> AFQETNPPAGPVRAIAEYERSAA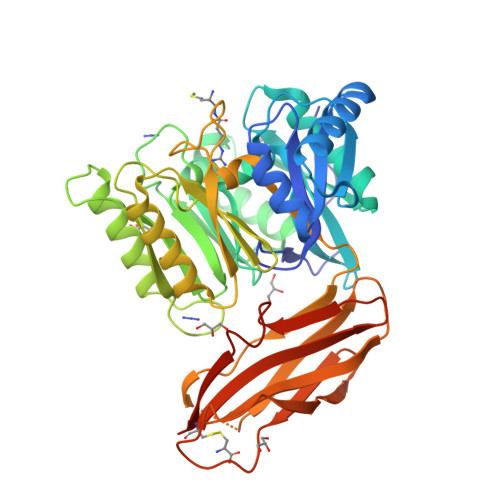VLVRYPFGIPMELIKELAKNDKVITIVASESQKNTVITQYTQSGVNLSNCDFIIAKTDSYWTRDYTGWFAMYDTNKVGLVDFIYNRPRPNDDEFPKYEAQYLGIEMFGMKLKQTGGNYMTDGYGSAVQSHIAYTENSSLSQAQVNQKMKDYLGITHHDVVQDPNGEYINHVDCWGKYLAPNKILIRKVPDNHPQHQALEDMAAYFAAQTCAWGTKYEVYRALATNEQPYTNSLILNNRVFVPVNGPASVDNDALNVYKTAMPGYEIIGVKGASGTPWLGTDALHARTHEVADKGYLYIKHYPILGEQAGPDYKIEADVVSCANATISPVQCYYRINGSGSFKAADMTMESTGHYTYSFTGLNKNDKVEYYISAADNSGRKETYPFIGEPDPFKFTCMNETNTCTVTGAA> DMLPEIAAAVGFLSSLLRTRGCVSEQRLKVFSRALQDALTDHYKHHWFPEKPSKGSGYR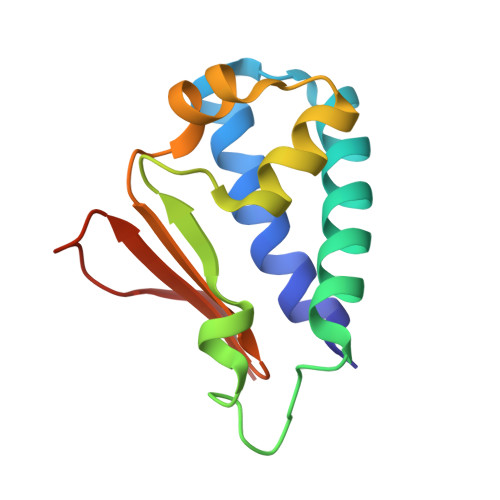CIRINHKMDPIISKVASQIGLSQPQLHRLLPSELTLWVDPYEVSYRIGEDGSICVLYEE ZER1 and ZYG11B, the substrate receptors of the Cullin 2-RING E3 ubiquitin ligase (CRL2), recognize N-terminal (Nt) glycine degrons and participate in the Nt-myristoylation quality control through the Gly/N-degron pathway. Here we show that ZER1 and ZYG11B can also recognize small Nt-residues other than glycine. Furthermore, we present the crystal structures of ZER1 and ZYG11B bound to various small Nt-residues and uncover the molecular mechanism of non-acetylated substrate recognition by ZER1 and ZYG11B. In conclusion, we propose that ZER1/ZYG11B not only targets Gly/N-degrons for proteasomal degradation, but it also has the ability to bind a defined selection of non-Ac/N-degrons by a conserved molecular mechanism of substrate recognition and target their degradation through the non-Ac/N-degron pathway.

To understand the molecular basis of ZER1/ZYG11B-mediated binding of non-Gly Nt-residue peptides, we determined the crystal structures of ZER1 bound to either SFLH-, AFLH- or TFLH-peptide, as well as the crystal structures of ZYG11B bound to either SFLH-, AFLH- or CFLH- peptide. Meanwhile, ZYG11B displayed appreciable binding to Nt-Ser (KD of 6.8), -Ala (KD of 7.1), or -Cys (KD of 3.0), albeit slightly weaker than Nt-Gly (KD of 2.5). Notably, ZER1 and ZYG11B also have the capacity to recognize the Nt-Cys, which is known to be only 50% Nt-acetylated by NatA in cells. GPS assays showed that in contrast to control GFP, the Cys-GFP fusion proteins are indeed efficiently degraded upon the overexpression of ZER1 or ZYG11B. Moreover, the Cys-GFP exhibited dramatic instability in response to NAA10 KD, whereas further double knock out of ZER1/ZYG11B was sufficient to restore Cys-GFP stability, establishing that the free Nt-Cys can be targeted by ZER1/ZYG11B for degradation. The free α-amino group of the Nt-residue forms hydrogen bonds with the side chains of Asp556 and Asn597 in ZER1 (the counterparts of Asp 526 and Asn 567 in ZYG11B), respectively. Furthermore, the carbonyl oxygen of the Nt-residue is stabilized by two hydrogen bonds from Asn597 and Trp552 in ZER1 (Asp 567 and Trp522 in ZYG11B). Likewise, consistent with the structural observations, the mutants W522A, D526A, N567A, E570A and N523A in ZYG11B were defective in binding to the XFLHVGQD (X = Ser, Ala or Cys) peptides.

>CFLHVGAQLGTELFIVRQLLQIVKQKTNQNSVDTTLKFTLSALWNLTDESPTTCRHFIENQGLELFMRVLESFPTESSIQQKVLGLLNNIAEVQELHSELMWKDFIDHISSLLHSVEVEVSYFAAGIIAHLISRGEQAWTLSRSQRNSLLDDLHSAILKWPTPECEMVAYRSFNPFFPLLGCFTTPGVQLWAVWAMQHVCSKNPSRYCSMLIEEGGLQHLYNIKDHEHTDPHVQQIAVAILDSLEKHIVR[2x]>[2x]MQKRAIYPGTF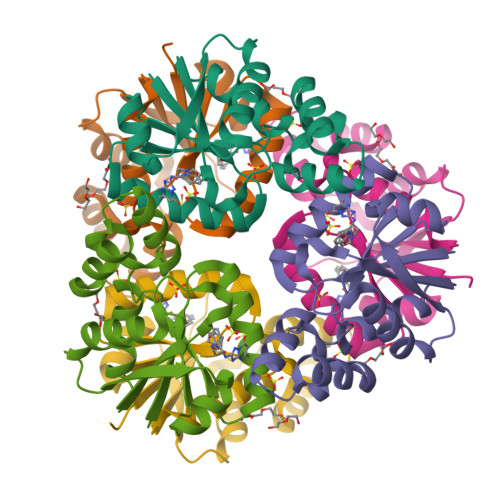DPITNGHIDIVTRATQMFDHVILAIAASPSKKPMFTLEERVALAQQATAHLGNVEVVGFSDLMANFARNQHATVLIRGLRAVADFEYEMQLAHMNRHLMPELESVFLMPSKEWSFISSSLVKEVARHQGDVTHFLPENVHQALMAKLAVD> MALKKEGPEFDHDDEVLLLEPGIMLDESSADEQPSPRATPKATTSFSSKQHKHIDYTRALDATQLYLNEIGFSPLLTPEEEVHFARLAQKGDPAGRKRMIESNLRLVVKIARRYVNRGLSLLDLIEEGNLGLIRAVEKFDPERGFRFSTYATWWIRQTIE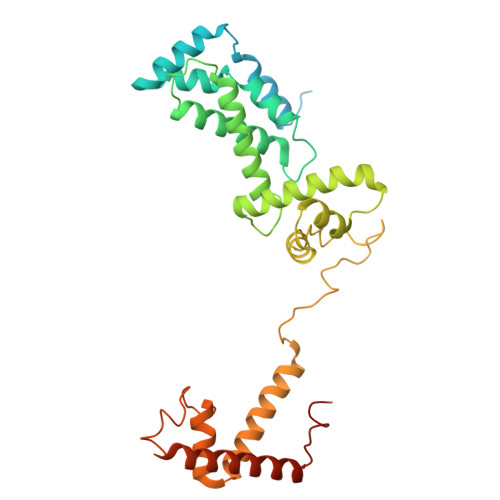RAIMNQTRTIRLPIHVVKELNVYLRAARELTHKLDHEPSPEEIANLLEKPVAEVKRMLGLNERVTSVDVSLGPDSDKTLLDTLTDDRPTDPCELLQDDDLSESIDQWLTELTDKQREVVIRRFGLRGHESSTLEEVGQEIGLTRERVRQIQVEALKRLREILEKNGLSSDALFQLEHHHHHH>[6x]ATPWQKITQPVPGSAQSIGSFSNGCIVGADTLPIQSEHYQVMRTDQRRYFGHPDLVMFIQRLSSQVSNLGMGTVLIGDMGMPAGGRFNGGHASHQTGLDVDIFLQLPKTRWTSAQLLRPQALDLVSRDGKHVVSTLWKPEIF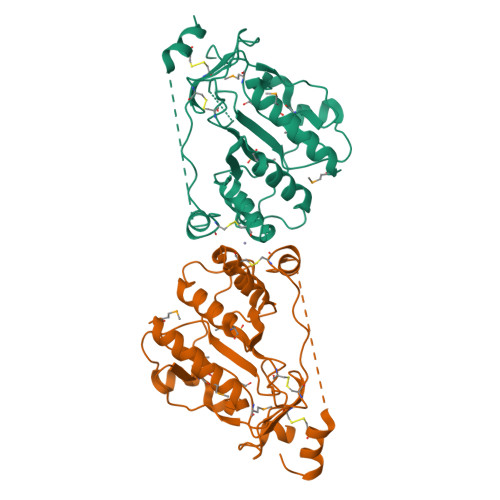SLIKLAAQDKDVTRIFVNPAIKQQLCLDAGTDRDWLRKVRPWFQHRAHMHVRLRCPADSLECEDQPLPPSGDGCGAELQSWFEPPKPGTTKPEKKTPPPLPPSCQALLDEHVI> GSFSREYTAAVEAKQVAQQEAQRAQFLVEKAKQEQRQKIVQAEG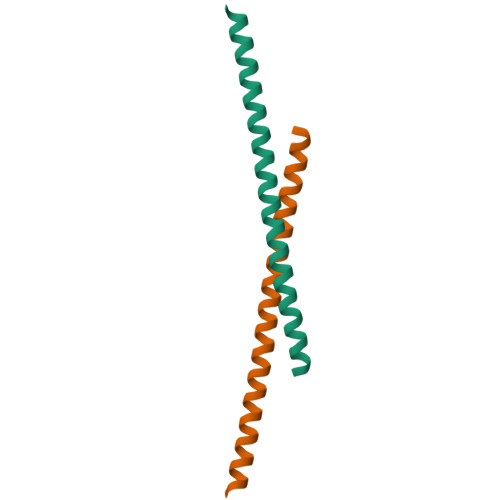EAEAAKMLGEALSKNPGYIKLRKIRAAQNISKTIALEHHHHHH> TRDETSIESFLGRSGCIAMIEFNTSSDKTEHDKIGKGFKTWKVSLQEMAQIRRKYELFTYTRFDSEITIVTAAAAQGNDSGHIVL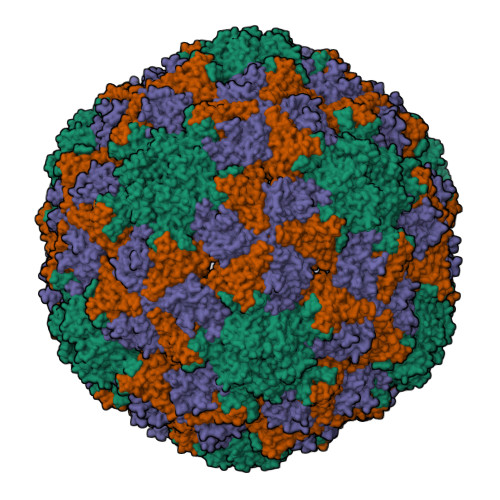QFMYVPPGAPVPEKRDDYTWQSGTNASVFWQEGQPYPRFTIPFMSIASAYYMFYDGYDGDSAASKYGSVVTNDMGTICVRIVTSNQKHDSNIVCRIYHKAKHIKAWCPRPPRAVAYQHTHSTNYIP;> IQITRGDSTITSQDTANAVVAYGVWPSYLTPDDATAIDKPTQPDTSSNRFYTLDSRSWTSASSGWWWKLPDALKNMGIFGENMFYHFLGRSGYTIHVQCNSSKFHQGLLIVAAIPEHQLASATSGNVSVGYNHTHPGEQGREVVPSRTSSDNKRPSDDSWLNFDGTLLGNLPIYPHQYINLRTNNSATLILPYVNAVPMDSMLRHNNWSLVIIPICPLQVQPGGTQSIPITVSISPMFSEFSGPRS;> PVMLTPGSGQFLTTDDTQSPSAFPYFHPTKEIFIPGQVRNLIEMCQVDTLIPVNNTQENVRSVNMYTVDLRTQVDLAKEVFSIPVDIASQPLATTLIGELASYYTHWTGSLRFSFMFCGSASSTLKLLIAYTPPGVGKPKSRREAMLGTHLVWDVGLQSTASLVVPWVSASHFRFTTPDTYSSAGYITCWYQTNFVVPDSTPDNAKMVCMVSACKDFCLRLARDTNLHT>[4x]MEEDKLALGREIFLERSEPQCALCHTLADAEAVGEVGPNLDELKPDAERVNTAVTN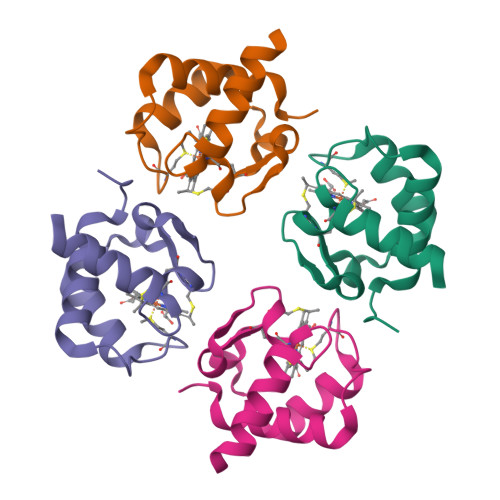GIGPMPANEILTDEEIEAVALYVSTVAGKAKNSSSVDKLAAALEHHHHHH>ADPGDQNPQIAAHVISEASSKTTSVLQWAEKGYYTMSNNLVTLENGKQLTVKRQGLYYIYAQVTFCSNREASSQAPFIASLCLKSPGRFERILLRAANTHSSAKPCGQQSIHLGGVFELQPGASVFVNVTDPSQVSHGTGFTSFGLLKL[6x];>EPPTACREKQYLINSQCCSLCQPGQKLVSDCTEFTETECLPCGESEFLDTWNRETHCHQHKY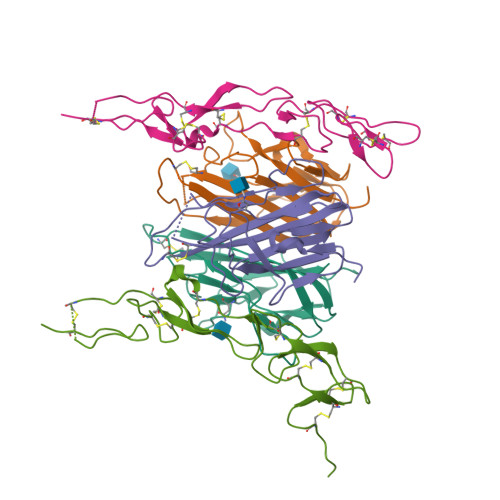CDPNLGLRVQQKGTSETDTICTCEEGWHCTSEACESCVLHRSCSPGFGVKQIATGVSDTICEPCPVGFFSNVSSAFEKCHPWTSCETKDLVVQQAGTNKTDVVCGPQDSGRLVPR[4x]>MPGGLLLGDVAPNFEANTTVGRIRFHDFLGDSWGILFSHPRDFTPVCTTELGRAAKLAPEFAKRNVKLIALSIDSVEDHLAWSKDINAYNCEEPTEKLPFPIIDDRNRELAILLGMLDPAEKDEKGMPVTARVVFVFGPDKKLKLSILYPATTGRNFDEILRVVISLQLTAEKRVATPVDWKDG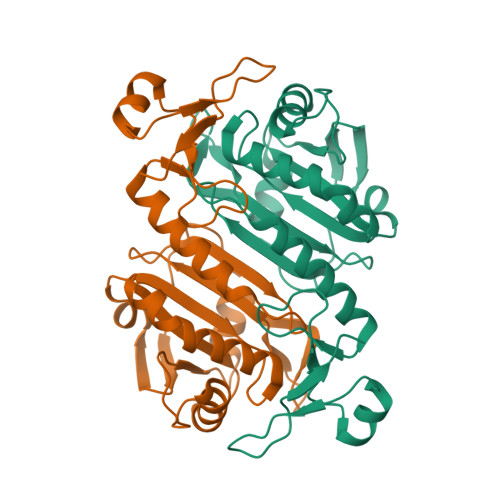DSVMVLPTIPEEEAKKLFPKGVFTKELPSGKKYLRYTPQP[6x]>[2x]MHHHHHHENLYFQGQHAQPPPQPRKKRPEDFKFGKILGEGSFSTVVLARELATSREYAIKILEKRHIIKENKVPYVTRERDVMSRLDHPFFVKLYFTFQDDEKLYFGLSYAKNGELLKYIRKIGSFDETCTRFYTAEIVSALEYLHGKGIIHRDLKPENILLNEDMHIQITDFGTAKVLSPE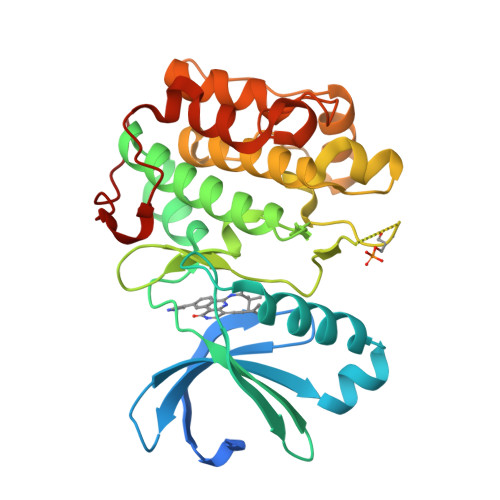SKQARANSFVGTAQYVSPELLTEKSACKSSDLWALGCIIYQLVAGLPPFRAGNEYLIFQKIIKLEYDFPEKFFPKARDLVEKLLVLDATKRLGCEEMEGYGPLKAHPFFESVTWENLHQQTPPKLTAYL>[2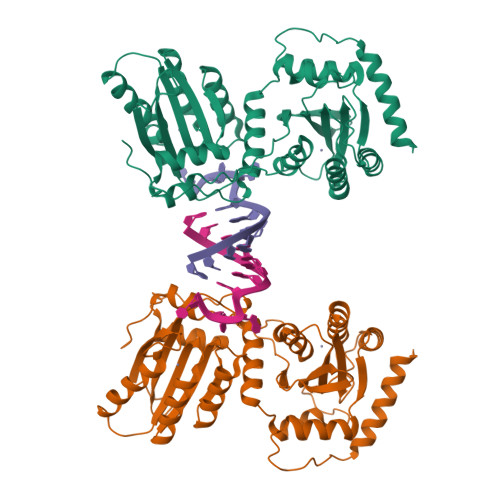x]GPGGSGGMKPQIRNMVEPMDPRTFVSNFNNRPILSGLDTVWLCCEVKTKDPSGPPLDAKIFQGKVYPKAKYHPEMRFLRWFHKWRQLHHDQEYKVTWYVSWSPCTRCANSVATFLAKDPKVTLTIFVARLYYFWKPDYQQALRILAEAGATMKIMNYNEFQDCWNKFVDGRGKPFKPWNNLPKHYTLLQATLGELLRHLMDPGTFTSNFNNKPWVSGQHETYLCYKVERLHNDTWVPLNQHRGFLRNQAPNIHGFPKGRHAALCFLDLIPFWKLDGQQYRVTCFTSWSPCFSCAQEMAKFISNNEHVSLCIFAARIYDDQGRYQEGLRTLHRDGAKIAMMNYSEFEYCWDTFVDRQGRPFQPWDGLDEHSQALSGRLRAILQNQGN>[4x]MDSTKAQTPEEQRAKNAKTILEN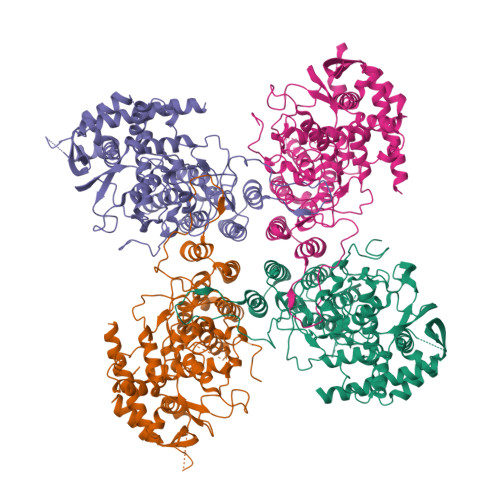IQIYERMCDLFGVSEDDKLIIENSISIERMIRVVTDKKYQDKKLKNAGSDLEKIANAGKVFCRLVESTAGKCSARLGMALKPNVEAVLTDVLGNELDRAAVLGKRMGFTAMFKSNLEEVLYQRGKNQLKKRNSAETFTLSQGASLEARFRPIMEKHLGVGTVVASIKNILASKKNGNYKNKMVRKPGGNRESWSPLEREISFLNKKLFPGPMRQLCKKFEYLNDQEKQLALNLMLDASLILKPQVTHKMIMPWSMWLAVKKYAEMNKGSPSLEDLAAYSGVRAFMAFNTACYMSKFTIGKGIVGDAEIMENGNDKMQILAMACFGLAYEDTGIVAAMISQPMKKRYQLKVGNFNPPEEGTIKGTSAGYFHKWAEFGNRLPFNSFGTGESKQISNSGVFAVQRPSTTNIQRLAELMARNTGETSDNFTQLVQKIREQVGTFADQKANLREFTGGYIYDITDVTKSNPKIPQLGGNSFFFEFTGSDVPRTGAKRRVGGADDVTLGTSQPKKRGRQGAGVESSMDIETVGED N-({(2Z)-2-[(4-hydroxyphenyl)methylidene]hydrazino}carbonothioyl)-beta-D-glucopyranosylamine 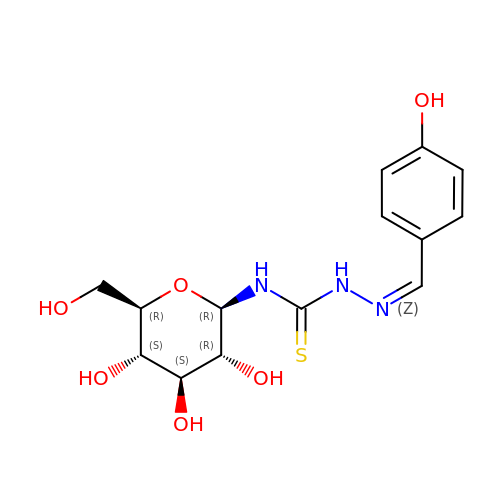| C14 H19 N3 O6 S | QWGDGYDWAFWBHA-ARDSGTFASA-N>MGPSLDFALSLLRRNVRQVQTDQGHFTMLGVRDRLAVLPRHSQPGKTIWIEHKLVNILDAVELVDEQGVNLELTLITLDTNEKFRDITKFIPENISTASDATLVINTEHMPSMFVPVGDVVQYGFLNLSGKPTHRTMMYNFPTKAGQCGGVVTSVGKVIGIHIGGNGRQGFCAGLKRSYFAS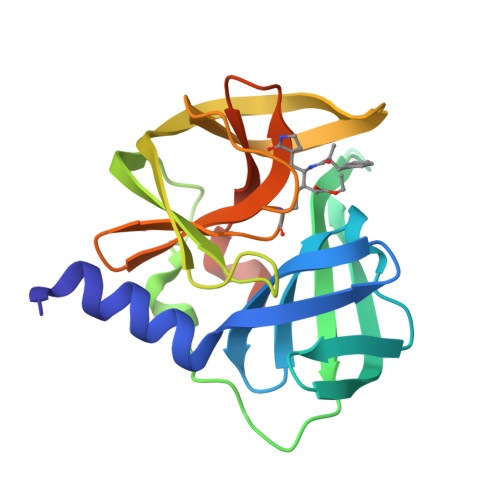EQLEHHHHHH[4x]> MGDEYK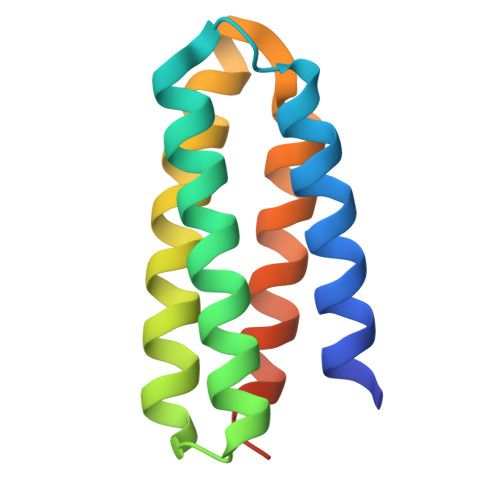KYYQQAIQLIQQLKKALEGNPEMKKLADKVLALLKQAYAAFKAGRSPEEIRALLRKAIEAAKKLAKLGASLGGFDLAKRIIELLKKMYELGGLEHHHHHH> GETSVPPGSALVGPSC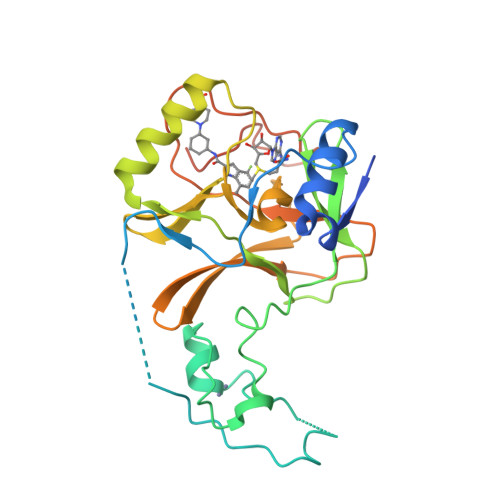VMDDFRDPQRWKECAKQGKMPCYFDLIEENVYLTERKKNKSHRDIKRMQCECTPLSKDERAQGEIACGEDCLNRLLMIECSSRCPNGDYCSNRRFQRKQHADVEVILTEKKGWGLRAAKDLPSNTFVLEYCGEVLDHKEFKARVKEYARNKNIHYYFMALKNDEIIDATQKGNCSRFMNHSCEPNCETQKWTVNGQLRVGFFTTKLVPSGSELTFDYQFQRYGKEAQKCFCGSANCRGYLGGENRVSIRAAGGKMKKERSRK>MFENITAAPADPILGLADLFRADERPGKINLGIGLYYDETGKIPVLTSVKKAEQYLLENETTKLYLGIDGIPEFGRCTQELLFGKGSALINDKRARTAQTPGGSGALRVAADFLAKNTSVKRVWVSNPSWPNHKSVFNSAGLEVREYAYYDAENHTLDFDALINSLNEAQAGDVVLFHGCCHNPTGIDPTLEQWQTLAQLSVEKGWLPLFDFAYQGFARGLEEDAEGLRAFAAMHKELIVASSYSKNFGLYNERVGACTLVAADSETVDRAFSQMKAAIRANYSSPPAHGASVVATILSNDALRAIWEQELTDMRQRIQRMRQLFVNTLQEKGANRDFSFIIKQNGMFSFSGLTKEQVLRLREEFGVYAVASGRVNVAGMTPDNM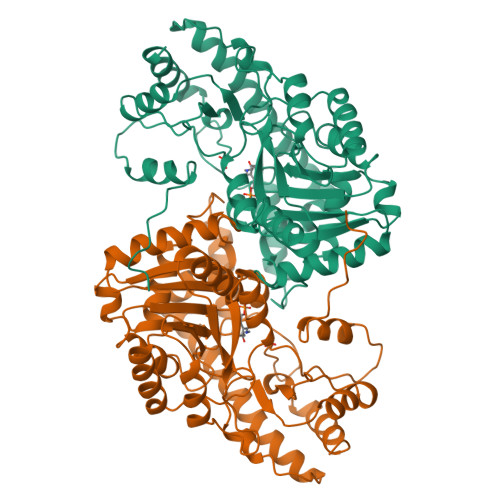APLCEAIVAVL[2x]>RADPDPMKNTCKLLVVADHRFYRYMGRGEESTTTNYLIELIDRVDDIYRNTAWDNAGFKGYGIQIEQIRILKSPQEVKPGEKHYNMAKSYPNEEKDAWDVKMLLEQFSFDIAEEASKVCLAHLFTYQDFDMGTLGLAYGGSPRANSHGGVCPKAYYSPVGKKNIYLNSGLTSTKNYGKTILTKEADLVTTHELGHNFGAEHDPDGLAECAPNEDQGGKYVMYPIAVSGDHENNKMFSQCSKQSIYKTIESKAQECFQERSNKVGSHHHHHH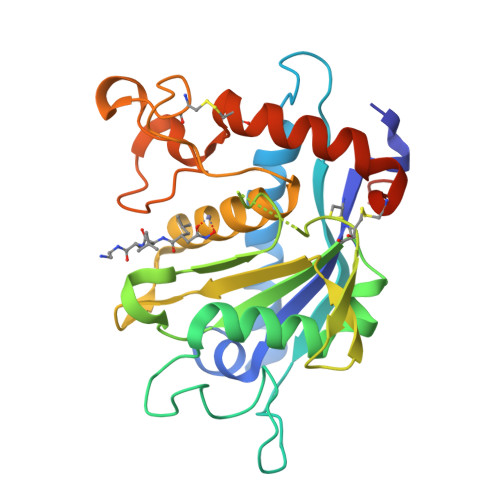[2x]We studied one type III effector from plant pathogenic bacteria called Pseudomonas syringae. This effector, termed avirulence protein B (AvrB), is targeted to the inner face of the plant cell plasma membrane, where it interacts with a membrane-bound host protein called RIN4 (resistance to Pseudomonas maculicula protein–interacting protein). A crystal structure of free AvrB revealed that it adopts a novel bilobal fold with no structural homologies to previously characterized proteins or functional domains. The junction of the two lobes forms a large solvent-accessible cleft with a volume of over 900 Å3 that extends into the lower lobe to form a pocket rich in conserved residues. Our data significantly extend previous observations defining the key functional regions of the type III effector protein AvrB: its upper lobe and interlobal cleft mediate contact with the Arabidopsis target protein RIN4, and the lower lobe contains a pocket suitable for binding ADP or another similarly shaped molecule.

We therefore examined binding to nucleotides, including adenosine triphosphate (ATP), adenosine diphosphate (ADP), guanosine diphosphate, and nonhydrolyzable ATP and guanosine diphosphate analogs, by soaking these into AvrB crystals. We found that crystallized AvrB could bind ADP within the lower lobe pocket of the large cavity (referred to as the ADP pocket). Significant interactions with ADP involve AvrB residues Y65, R99, and R266. Y65 stacks below the adenine ring and hydrogen bonds to the 2-OH group of the ribose, while R99 and R266 form salt bridges with the alpha- and beta-phosphates, respectively. N62 and F113 also contact the adenine base and phosphates, respectively. The conserved AvrB residues Y131 and D297 located at the interlobe boundary are approximately 4 Å from ADP and appear to contact it only via bridging water molecules. Mutation of ADP-binding residues in AvrBY65A, AvrBR99A, and AvrBR266A resulted in complete loss of AvrB-induced RPM1 function. The requirement of ADP interacting residues for AvrB phosphorylation suggests that nucleotide binding by AvrB is critical for this event. By contrast, the important ADP-contacting residues Y65, R99, and R266 in the lower lobe pocket are conserved in all AvrB homologs, suggesting that nucleotide binding is a core function for this entire type III effector family. In the AvrB/ADP structure, we could not definitively observe a Mg2+ ion.

> GAMGCVSSKSTTVLSPQTSFNEASRTSFRALPGPSQRQLEVYDQCLIGAARWPDDSSKSNTPENRAYCQSMYNSIRSAGDEISRGGITSFEELWGRATEWRLSKLQRGEPLYSAFASERTSDTDAVTPLVKPYKSVLARVVDHEDAHDEIMQDNLFGDLNVKVYRQTAYLHGNVIPLNTFRVATDTEYLRDRVAHLRTELGAKALKQHLQRYNPDRIDHTNASYLPIIKDHLNDLYRQAISSDLSQAELISLIARTHWWAASAMPDQRGSAAKAEFAARAIASAHGIELPPFRNGNVSDIEAMLSGEEEFVEKYRSLLDSDCF> AMSAIKPDMRIKLRMEGNVNGHHFVIDGDGTGKPYEGKQTMDLEVKEGGPLPFAFDILTTAFHYGNRVFVKYPDNIQDYFKQSFPKGYSWERSMTFEDGGICNARNDITMEGDTFYNKVRFYGTNFPANGPVMQKKTLKWEPSTEKMYVRDGVLTGDIEMALLLEGNAHYRCDFRTTYKAKEKGVKLPGAHFVDHAIEILSHDKDYNKVKLYEHAVAHSG

Photoconvertible fluorescent proteins (PCFPs) are commonly employed in super‐resolution microscopy techniques such as Photo‐Activated Localization Microscopy (PALM), single‐particle‐tracking PALM (sptPALM) and more recently MINFLUX (Balzarotti et al., 2017). We systematically characterized the maturation speed of mEos‐derived PCFPs in Escherichia coli and found that, in contrast to pcStar and mEosEM, several variants such as mEos2, mEos3.1, mEos3.2, and mEos4b mature extremely slowly. In this work, we present a comprehensive investigation of the maturation speed of PCFPs from the mEos family and propose strategies to considerably reduce the maturation time of the monomeric, bright, and fixation‐resistant mEos4b variant (Paez‐Segala et al., 2015). Through a structure‐guided mutagenesis strategy, we developed a strategy to reduce the day‐long maturation time of mEos4b by nearly two orders of magnitude without significantly impacting its molecular brightness and photophysical performance under single‐molecule imaging conditions.

Similarly, we hypothesized that the L93M mutation, which distinguishes mEos3.2 from pcStar and mEos4b from mEosEM, could be pivotal in the significant reduction in maturation time observed for pcStar and mEosEM. In contrast, the L93M mutant showed a drastically decreased apparent maturation time of approximately 80 min, a more than 20‐fold improvement relative to the mEos4b parent and better than any other L93 substitution we have tested. Despite this improvement, the maturation rate of mEos4b‐L93M remained approximately three‐fold slower compared to that of pcStar or mEosEM, both of which also have a methionine at position 93. As a first step towards further improvements, we sought to understand the rationale behind the observed accelerated maturation for mEos4b‐L93M. The only significant difference (beside the L93M mutation) was the presence of an extra water molecule in the vicinity of the chromophore, which is well ordered as evidenced by the clear electron density map at this position. This water molecule (W1 hereafter) is within hydrogen‐bonding distance of the sulfur atom of M93 and the hydroxyl group of T59. First, the L93M mutation enlarges a hydrophobic pocket adjacent to the chromophore and stabilizes a single ordered water molecule (W1) that bridges T59 and R91, subtly repositioning the catalytic arginine. In both computed structural models, the amide group of Q60 replaces the water molecule W1 observed in the mEos4b‐L93M structure, leading to a similar repositioning of the R91 side chain relative to T59. Significant acceleration of mEos4b maturation was achieved by modifying the immediate environment of R91, a residue known to play a key role in catalyzing maturation.>[2x]SNAMADEIAKAQVARPGGDTIFGKIIRKEIPAKIIFEDDRCLAFHDISPQAPTHFLVIPKKHISQISVAEDDDESLLGHL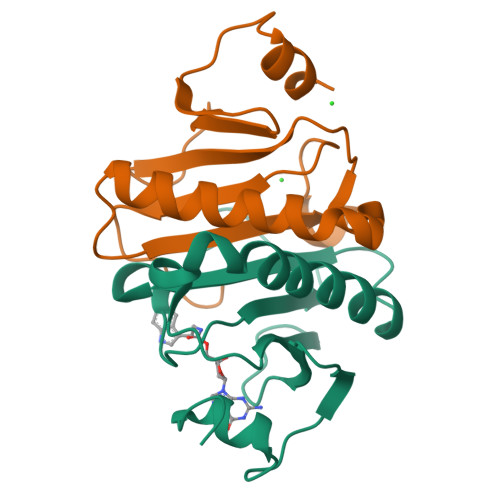MIVGKKCAADLGLNKGYRMVVNEGSDGGQSVYHVHLHVLGGRQMHWPPG> ACDYTCGSNCYSSSDVSTAQAAGYKLHEDGETVGSNSYPHKYNNYEGFDFSVSSPYYEWPILSSGDVYSGGSPGADRVVFNEN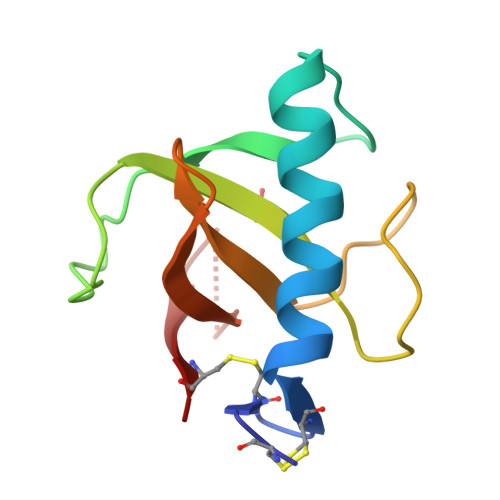NQLAGVITATGASGNNFVECT> MSAIKPDMKIKLRMEGNVNGHHFVIDGDGTGKPFEGKQSMDLEVKEGGPLPFAFDILTTAFXNRVFAKYPDNIQDYFKQSFPKGYSWERSLTFEDGGICNARNDITMEGDTFYNKVRFYGTNFPANGPVMQKKTLKWEPSTEKMYVRDGVLTGDVETALLLEGNAHYRCDFRTTYKAKEKGV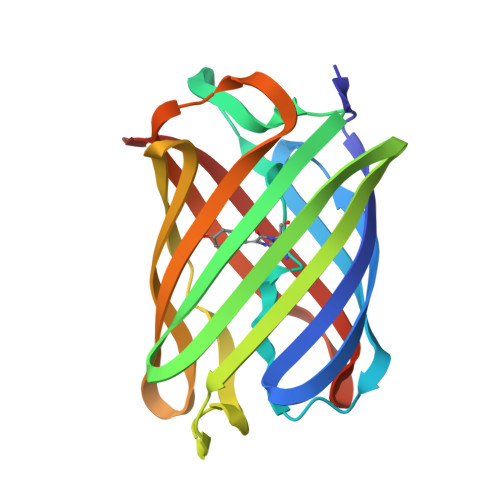KLPGAHFVDHCIEILSHDKDYNKVKLYEHAVAHSGLPN>[3x]GAMGSLIRKKAAGLESAATIRTKVFVWGLNDKDQLGGLKGSKIKVPSFSETLSALNVVQVAGGSKSLFAVTVEGKVY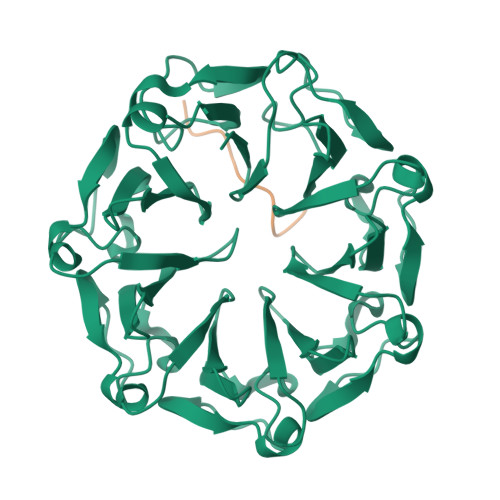ACGEATNGRLGLGISSGTVPIPRQITALSSYVVKKVAVHSGGRHATALTVDGKVFSWGEGDDGKLGHFSRMNCDKPRLIEALKTKRIRDIACGSSHSAALTSSGELYTWGLGEYGRLGHGDNTTQLKPKMVKVLLGHRVIQVACGSRDAQTLALTDEGLVFSWGDGDFGKLGRGGSEGCNIPQNIERLNGQGVCQIECGAQFSLALTKSGVVWTWGKGDYFRLGHGSDVHVRKPQVVEGLRGKKIVHVAVGALHCLAVTDSGQVYAWGDNDHGQQGNGTTTVNRKPTLVQGLEGQKITRVACGSSHSVAWTTVDVATPSVHEPVLFQT;>GFDEDKDEDEGSPGG[3x]> MDFYQLPGSPPCRAV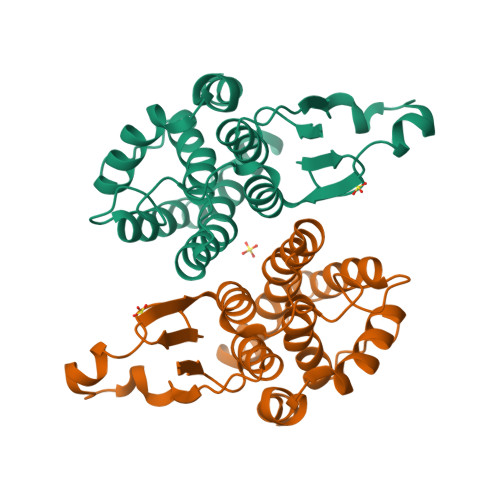ALTAAALDIEMNFKQVNLMNGEHLKPEFLKINPQHTIPTIDDNGFRLWESRAIMTYLADQYGKNDTLYPKDLKKRAIVNQRLYFDMSSLYKSFMDYYYPIIFMKAVKDQAKYENIGTALSFLDKFLEGENYVAGKNMTLADLSIVSTVSTLEALDYDLSKYKNVTRWFAKIKPEIPKYEEYNNAGLKMFKELVNEKLSKK> TPLVHVASVEKGRSYEDFQKVYNAIALKLREDDEYDNYIGYGPVLVRLAWHTSGTWDKHDNTGGSYGGTYRFKKEFNDPSNAGLQNGFKFLEPIHKEFPWISS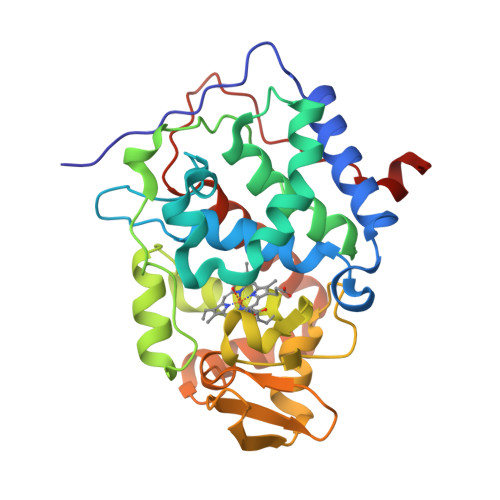GDLFSLGGVTAVQEMQGPKIPWRCGRVDTPEDTTPDNGRLPDADKDADYVRTFFQRLNMNDREVVALMGAHALGKTHLKNSGYEGPWGAANNVFTNEFYLNLLNEDWKLEKNDANNEQWDSKSGYMMLPTDYSLIQDPKYLSIVKEYANDQDKFFKDFSKAFEKLLENGITFPKDAPSPFIFKTLEEQGL Here we present the high-resolution cryo-EM structure of amyloid fibrils of the Src-homology 3 domain of phosphatidyl-inositol-3-kinase (PI3K-SH3). The structure of natively folded PI3K-SH3, a domain consisting of 86 amino acids from bovine PI3K, has been well-characterised by X-ray crystallography and NMR spectroscopy. SH3 domains are known to play a significant role in several signalling pathways where they mediate protein-protein interactions by recognising PxxP sequence motifs. Used initially as a model system for protein folding studies, PI3K-SH3 was among the first proteins discovered to form amyloid fibrils in the test tube, while not being associated to any known human disease.

A three-dimensional density map for the thick PI3K-SH3 fibril could be reconstructed to an overall resolution of 3.4 Å. The clear density of the fibril allowed us to build an atomic model for residues 1–77 out of a total of 86 amino acids. The missing nine residues are located at the C-terminus, which shows blurred density likely due to substantial flexibility. The thick PI3K-SH3 fibril is a left-handed helical structure consisting of two intertwined protofilaments, and is thus called DF (double filament) fibril. Protofilament subunits (PI3K-SH3 monomers) are stacked in a parallel, in-register cross-β structure. The helical symmetry is therefore described by a twist of 179.4 ° and rise of 2.35 Å, which corresponds to an approximate 21-screw symmetry. Each protofilament subunit, or PI3K-SH3 monomer, consists of seven parallel in-register β-strands (β1, aa1-5; β2, aa7-19; β3, aa22-26; β4, aa28-34; β5, aa46-56; β6, aa59-68; β7, aa72-77) that are interrupted by either sharp kinks, glycine or proline residues—or a combination of those. By encompassing 13 residues of each monomer, 26 in total, the inter-filament interface of the PI3K-SH3 DF fibril is very large. The protofilaments mainly interact through two identical symmetry-related hydrophobic patches at the periphery of their interface, between the bottom part of the bent β-arch motif and the respective C-terminal part of the opposing protofilament. A single subunit in the PI3K-SH3 DF fibril is not planar but winds itself along the protofilament axis, which leads to interlocking within a protofilament.

>[7x]GSMSAEGYQYRALYDYKKEREEDIDLHLGDILTVNKGSLVALGFSDGQEAKPEEIGWLNGYNETTGERGDFPGTYVEYIGRKKISP> GCAT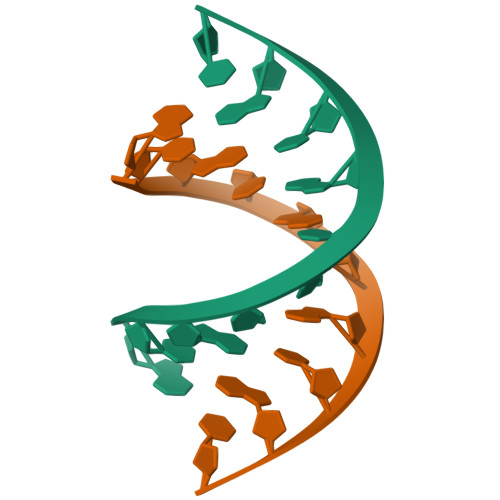GCATGC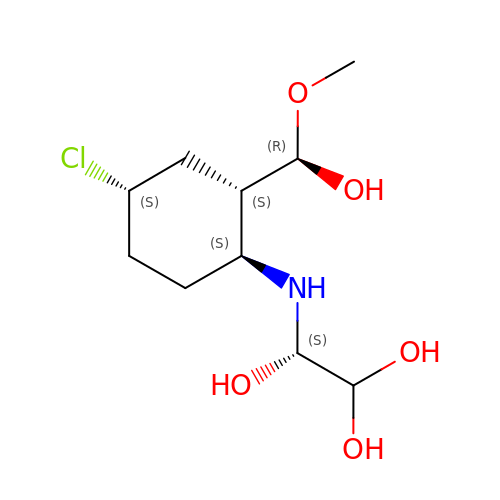2-({4-CHLORO-2-[HYDROXY(METHOXY)METHYL]CYCLOHEXYL}AMINO)ETHANE-1,1,2-TRIOL | C10 H20 Cl N O5 | ZCXQIUYGWAQWDL-MOQQMVQXSA-N>XGEVAQAVKEVAKAVKEVAWAVKEVAQAVKG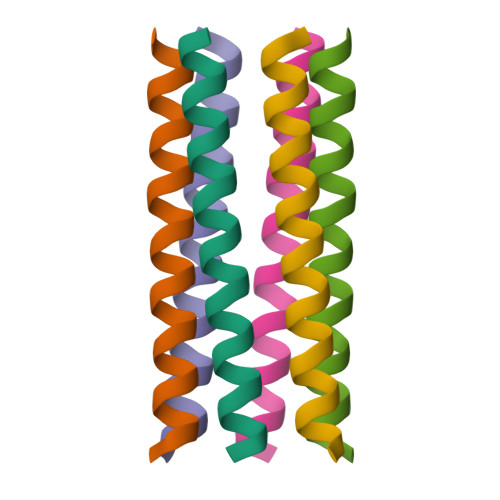X[12x]>[4x]GAMDPSPNYDKWEMERTDITMKHKLGGGQYGEVYEGVWKKYSLTVAVKTLKEDTME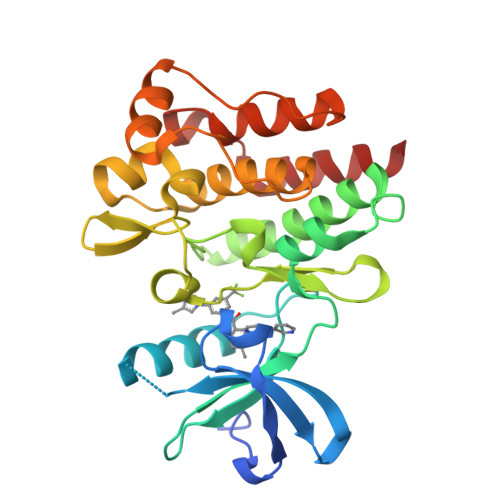VEEFLKEAAVMKEIKHPNLVQLLGVCTREPPFYIITEFMTYGNLLDYLRECNRQEVNAVVLLYMATQISSAMEYLEKKNFIHRDLAARNCLVGENHLVKVADFGLSRLMTGDTYTAHAGAKFPIKWTAPESLAYNKFSIKSDVWAFGVLLWEIATYGMSPYPGIDLSQVYELLEKDYRMERPEGCPEKVYELMRACWQWNPSDRPSFAEIHQAFETMFQES>[2x]DRRSFSSRTPVNENPDGVQYRRGFVTRHQVSGWRFVMRRIASGVALHDTRMLVDPLRTQSRAVLTGALILVTGLVGCFIFSLF;>[4x]PIVRVAVLAAGDDGGRLTEMALPSELPLREILPAVQRIVQPARENDGAADPAAAPNPVRLSLAPIGGAPFSLDATLDTVGVVDGDLLALQAVPSGPPAPRIVEDIADAAVIFSEARRRQWGPTHIARGAALALIGLILVGTGLSVAHRVITGDLLGQFIVSGIALATVIAALAVRNRSAVLATSLAVTALVPVAAAFALGVPGDFGAPNVLLAAAGVAAWSLISMAGSPDDRGI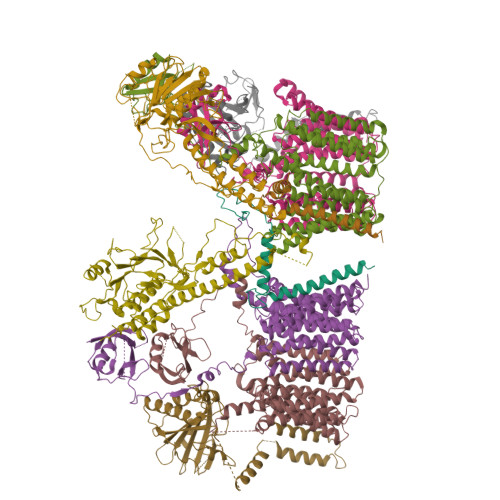AVFTATAVTGVGVLLVAGAASLWVISSDVIGCALVLLGLIVTVQAAQLSAMWARFPLPVIPAPGDPTPAARPLSVLADLPRRVRVSQAHQTGVIAAGVLLGVAGSVALVSSANASPWAWYIVVAAAAGAALRARVWDSAACKAWLLGHSYLLAVALLVAFVIGDRYQAALWALAALAVLVLVWIVAALNPKIASPDTYSLPMRRMVGFLATGLDASLIPVMALLVGLFSLV;>[2x]MTARIALASLFVVAAVLAQPWQTTTQRWVLGVSIAAVIVLLAWWKGMFLTTRIGRALAMVRRNRAEDTVETDAHRATVVLRVDPAAPAQLPVVVGYLDRYGITCDKVRITHRDAGGTRRSWISLTVDAVDNLAALQARSARIPLQDTTEVVGRRLADHLREQGWTVTVVEGVDTPLPVSGKETWRGVADDAGVVAAYRVKVDDRLDEVLAEIGHLPAEETWTALEFTGSPAEPLLTVCAAVRTSDRPAAKAPLAGLTPARGRHRPALAALNPLSTERLDGTAVPL;>SRLIFEHQRRLTPPTTRKGTITIEPPPQLPRVVPPSLLRRVLPFLIVILIVGMIVALFATGMRLISPTMLFFPFVLLLAATALYRGGDNKMRTEEVDAERADYLRYLSVVRDNVRAHAAEQRAALEWSHPEPEVLATIPGTRRQWERDPRDRDFLVLRAGRHDVPLDAALKVKDTADEIDLEPVAHSALRGLLDVQRTVRDAPTGLDVAKLARITVIGEADEARAAIRAWIAQAVTWHDPTMLGVALAAPDLESGDWSWLKWLPHVDVPNEADGVGPARYLTTSTAELRERLAPALADRPLFPAESGAALKHLLVVLDDPDADPDDIARKPGLTGVTVIHRTTELPNREQYPDPERPILRVADGRIERWQVGGWQPCVDVADAMSAAEAAHIARRLSRWDS[2x]>[2x]SLFELGKMILQETGKNPAKSYGAYG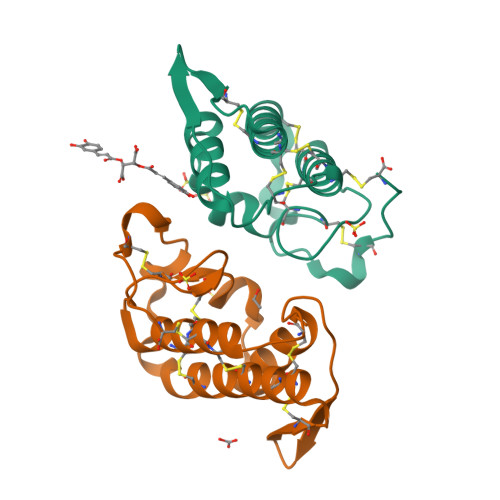CNCGVLGRGKPKDATDRCCYVHKCCYKKLTGCNPKKDRYSYSWKDKTIVCGENNPCLKELCECDKAVAICLRENLGTYNKKYRYHLKPFCKKADPC pelargonidin 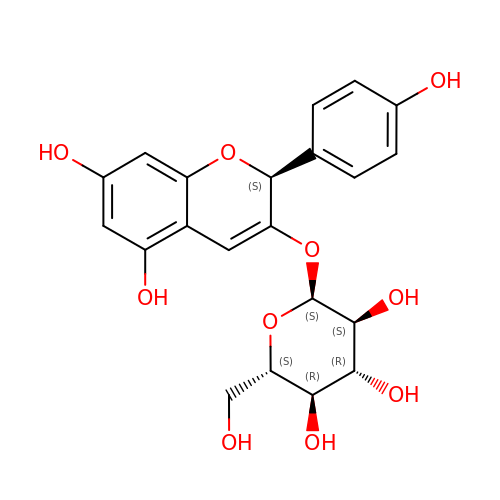3-O-beta-D-glucoside | C21 H22 O10 | SNGNSJWVINEVCL-FGWZRKRKSA-N> GSSFVHLHNHTEYSMLDGAAKITPMLAEVERLGMPAVGMTDHGNMFGASEFYNSATKAGIKPIIGVEAYIAPGSRFDTRRILWGDPSQKADDVSGSGSYTHLTMMAENATGLRNLFKLSSHASFEGQLSKWSRMDAELIAEHAEGIIITTGCPSGEVQTRLRLGQDREALEAAAKWREIVGPDNYFLELMDHGLTIERRVRDGLLEIGRALNIPPLATNDCHYVTRDAAHNHEALLCVQTGKTLSDPNRFKFDGDGYYLKSAAEMRQIWDDEVPGACDSTLLIAERVQSYADVWTPRDRMPVFPVPDGHDQASWLRHEVDAGLRRRFPAGPPDGYRERAAYEIDVICSKGFPSYFLIVADLISYARSAGIRVGPGRGSAAGSLVAYALGITDIDPIPHGLLFERFLNPERTSMPDIDIDFDDRRRGEMVRYAADKWGHDRVAQVITFGTIKTKAALKDSARIHYGQPGFAIADRITKALPPAIMAKDIPLSGITDPSHERYKEAAEVRGLIETDPDVRTIYQTARGLEGLIRNAGVHACAVIMSSEPLTEAIPLWKRPQDGAIITGWDYPACEAIGLLKMDFLGLRNLTIIGDAIDNVRANRGIDLDLESVPLDDKATYELLGRGDTLGVFQ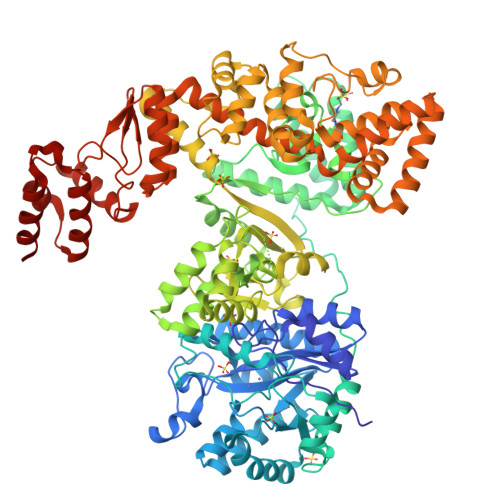LDGGPMRDLLRRMQPTGFEDVVAVIALYRPGPMGMNAHNDYADRKNNRQAIKPIHPELEEPLREILAETYGLIVYQEQIMRIAQKVASYSLARADILRKAMGKKKREVLEKEFEGFSDGMQANGFSPAAIKALWDTILPFADYAFNKSHAAGYGMVSYWTAYLKANYPAEYMAGLLTSVGDDKDKAAVYLADCRKLGITVLPPDVNESGLNFASVGQDIRYGLGAVRNVGANVVGSLLQTRNDKGKFTDFSDYLNKIDISACNKKVTESLIKAGAFDSLGHARKGLFLVHSDAVD>[4x]MGHHHHHHMGLFAGKGVLVTGGARGIGRAIAQAFAREGALVALCDLRPEGKEVAEAIGGAFFQVDLEDERERVRFVEEAAYALGRVDVLVNNAAIAAPGSALTVRLPEWRRVLEVNLTAPMHLSAL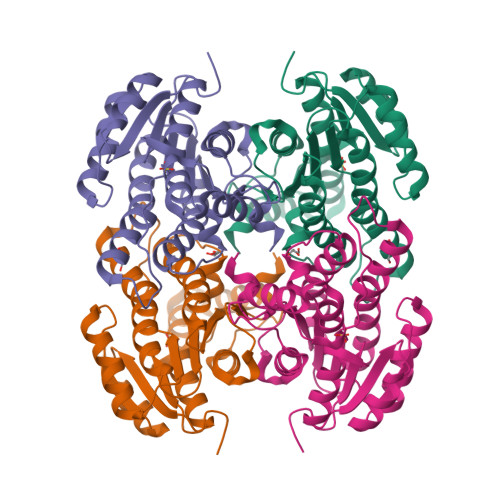AAREMRKPGPGAIVNVASYLGLFAEQENAAYNASKGGLVNLTRSLALDLAPLRIRVNAVAPGFIATEALLELIALSPDPERTRRDMEDLHALRRLGKPEEVAEAVLFLASEKASFITGAILPVDGGLTASFMMAGRPV> MAAHVESEFSFDLDHIEQVTSRARGFKEFVTENLDQLESRAQKLVQSGQWAGAAAAAYSQAHKEWMDAAREL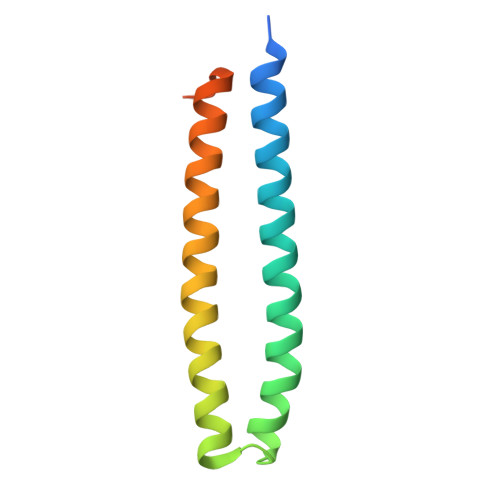VEGLSQMEEAARTAHGAYSEAQEANLRMARG> MHHHHHHKSNDMNITVELTFFEPYRLVEWFDWDARKKSHSAMRGQAFAQWTWKGKGRTAGKSFITGTLVRSAVIKAVEELLSLNNGKWEGVPCCNGSFQTDESKGKKPSFLRKRHTLQWQANNKNICDKEEACPFCILLGRFDNAGKVHERNKDYDIHFSNFDLDHKQEKNDLRLVDIASGRILNRVDFDTGKAKDYFRTWEADYETYGTYTGRITLRNEHAKKLLLASLGFVDKLCGALCRIEVIKKSESPLPSDTKEQSYTKDDTVEVLSEDHNDELRKQAEVIVEAFKQNDKLEKIRILADAIRTLRLHGEGVIEKDELPDGKEERDKGHHLWDIKVQGTALRTKLKELWQSNKDIGWRKFTEMLGSNLYLIYKKETGGVSTRFRILGDTEYYSKAHDSEGSDLFIPVTPPEGIETKEWIIVGRLKAATPFYFGVQQPSDSIPGKEKKSEDSLVINEHTSFNILLDKENRYRIPRSALRGALRRDLRTAFGSGCNVSLGGQILCNCKVCIEMRRITLKDSVSDFSEPPEIRYRIAKNPGTATVEDGSLFDIEVGPEGLTFPFVLRYRGHKFPEQLSSVIRYWEENDGKNGMAWLGGLDSTGKGRFALKDIKIFEWDLNQKINEYIKERGMRGKEKELLEMGESSLPDGLIPYKFFEERECLFPYKENLKPQWSEVQYTIEVGSPLLTADTISALTEPGNRDAIAYKKRVYNDGNNAIEPEPRFAVKSETHRGIFRTAVGRRTGDLGKEDHEDCTCDMCIIFGNEHESSKIRFEDLELINGNEFEKLEKHIDHVAIDRFTGGALDKAKFDTYPLAGSPKKPLKLKGRFWIKKGFSGDHKLLITTALSDIRDGLYPLGSKGGVGYGWVAGISIDDNVPDDFKEMINKTEMPLPEEVEESNNGPINNDYVHPGHQSPKQDHKNKNIYYPHYFLDSGSKVYREKDIITHEEFTEELLSGKINCKLETLTPLIIPDTSDENGLKLQGNKPGHKNYKFFNINGELMIPGSELRGMLRTHFEALTKSCFAIFGEDSTLSWRMNADEKDYKIDSNSIRKMESQRNPKYRIPDELQKELRNSGNGLFNRLYTSERRFWSDVSNKFENSIDYKREILRCAGRPKNYKGGIIRQRKDSLMAEELKVHRLPLYDNFDIPDSAYKANDHCRKSATCSTSRGCRERFTCGIKVRDKNRVFLNAANNNRQYLNNIKKSNHDLYLQYLKGEKKIRFNSKVITGSERSPIDVIAELNERGRQTGFIKLSGLNNSNKSQGNTGTTFNSGWDRFELNILLDDLETRPSKSDYPRPRLLFTKDQYEYNITKRCERVFEIDKGNKTGYPVDDQIKKNYEDILDSYDGIKDQEVAERFDTFTRGSKLKVGDLVYFHIDGDNKIDSLIPVRISRKCASKTLGGKLDKALHPCTGLSDGLCPGCHLFGTTDYKGRVKFGFAKYENGPEWLITRGNNPERSLTLGVLESPRPAFSIPDDESEIPGRKFYLHHNGWRIIRQKQLEIRETVQPERNVTTEVMDKGNVFSFDV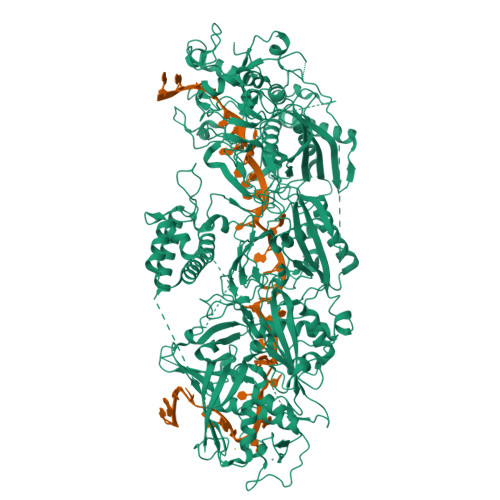RFENLREWELGLLLQSLDPGKNIAHKLGKGKPYGFGSVKIKIDSLHTFKINSNNDKIKRVPQSDIREYINKGYQKLIEWSGNNSIQKGNVLPQWHVIPHIDKLYKLLWVPFLNDSKLEPDVRYPVLNEESKGYIEGSDYTYKKLGDKDNLPYKTRVKGLTTPWSPWNPFQVIAEHEEQEVNVTGSRPSVTDKIERDGKMV> MRSDGRK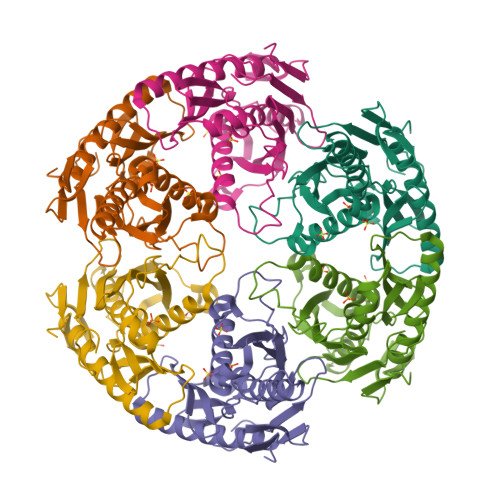EDQLRPVSIQRDFLEYPEGSCLISFGKTKVICTASVIENVPNWLKGKGQGWITAEYSMLPRATQQRTIRESVQGRIGGRTHEIQRMIGRAMRTAVELTKIGERTIWVDCDVIQADGGTRTAAITGAFVAVADAIIKLHKEGIIEETPIKDFVAAVSVGIVNDRILLDLNFEEDSAAQVDMNVVGTGSGRLSEVHTMGEEYSFTKDELIKMLDLAQKGINELIELQKKLYVIQDGKWERSELKEVSSTT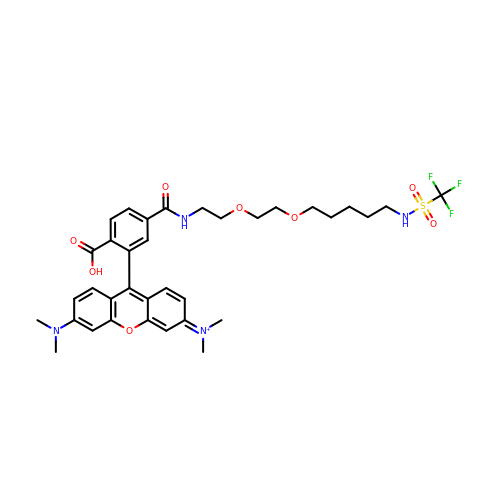[9-[2-carboxy-5-[2-[2-[5-(trifluoromethylsulfonylamino)pentoxy]ethoxy]ethylcarbamoyl]phenyl]-6-(dimethylamino)xanthen-3-ylidene]-dimethyl-azanium | C35 H42 F3 N4 O8 S | QNUHBXCAJKIQSP-UHFFFAOYSA-O> SNAMKKAVLIVNPSSGGEKAKEFETLAEEKLKQLFDEVVVKQTEKGGDAEQFAREAAESHFDSVFVMGGDGTVNEGISGLAEQAYRPKFGFFPLGTVNDLARALNLPMDPEEAIQQLDLEKTSALDVGKINDDYFMNVVAIGTIPESINDVDVEQKTKLGKLAYFISGAKHLANAQTYPFHLSLDQKEQTIESSTVLVGLTNSIGGFETLLPEAQVDDGKLHLVYLKDQSLWDAVKAVPDLLKGVDQSTDNLVYLTFKEGTISLENQEELTTNVDGDEG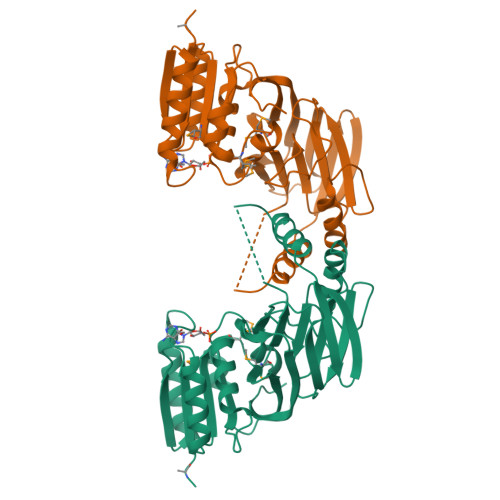AALPITLKILPKHLTVYCGEEQTK> MRCTHLENRDFVTGTQGTTRVTLVLELGGCVTITAEGKPSMDVWLDSIYQENPAKTREYCLHAKLSDTKVAARCPTMGPATLAEEHQSGTVCKRDQSDRGWGNHCGLFGKGSIVTCVKASCEAKKKATGHVYDANKIVYTVKVEPHTGDYVAANETHSGRKTASFTVSSERTI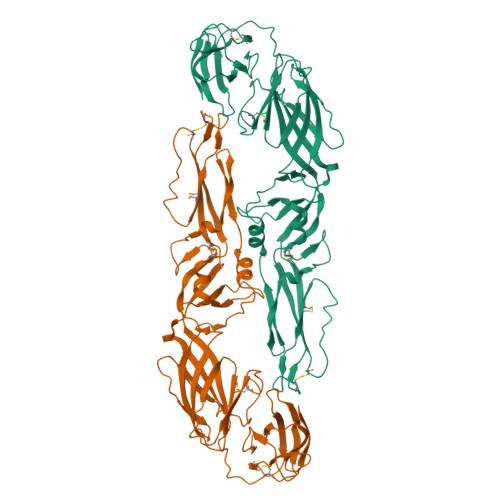LTMGDYGDVSLLCRVASGVDLAQTVILELDKTSEHLPTAWQVHRDWFNDLALPWKHEGAQNWNNAERLVEFGAPHAVKMDVYNLGDQTGVLLKSLAGVPVAHIDGTKYHLKSGHVTCEVGLEKLKMKGLTYTMCDKTKFTWKRIPTDSGHDTVVMEVAFSGTKPCRIPVRAVAHGSPDVNVAMLMTPNPTIENNGGGFIEMQLPPGDNIIYVGELSHQWFQK> MGSSHHHHHHGGGSENLYFQGSDQAALVNRTTLIDARRSEAMTNAALEMERSYRQYCVLDDPTLAKVYQSQRKRYSEMLDAHAGVLPDDKLYQALRQDLNNLAQLQCNNSGPDAAAAARLEAFASANTEMVQATRTVVFSRGQQL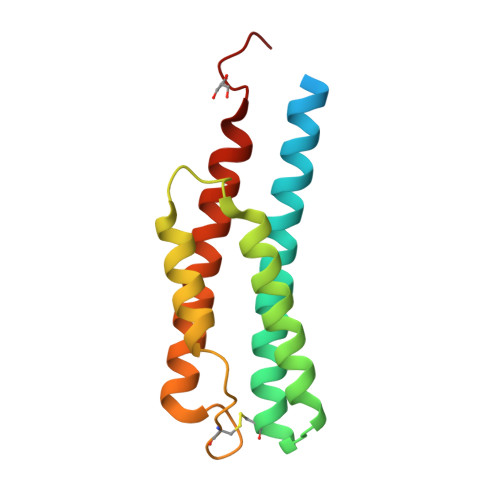QRE>[7x]MAIAQLATEYVFSDFLLKEPTEPKFKGLRLELAVDKMVTCIAVGLPLLLISLAFAQEISIGTQISCFSPSSFSWRQAAFVDSYCWAAVQQKNSLQSESGNLPLWLHKFFPYILLLFAILLYLPPLFWRFAAAPHICSDLKFIMEELDK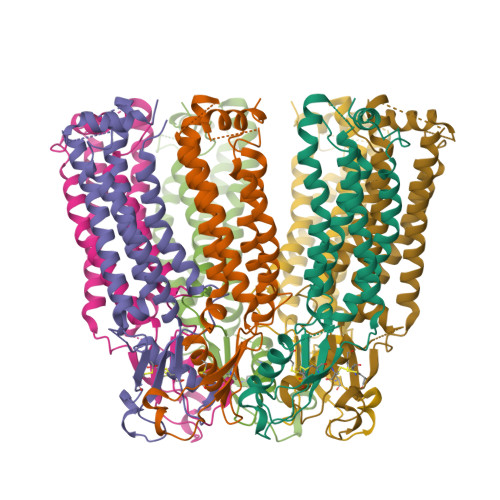VYNRAIKAAKSARDLDMRDGACSVPGVTENLGQSLWEVSESHFKYPIVEQYLKTKKNSNNLIIKYISCRLLTLIIILLACIYLGYYFSLSSLSDEFVCSIKSGILRNDSTVPDQFQCKLIAVGIFQLLSVINLVVYVLLAPVVVYTLFVPFRQKTDVLKVYEILPTFDVLHFKSEGYNDLSLYNLFLEENISEVKSYKCLKVLENIKSSGQGIDPMLLLTNLGMIKMDVVDGKTPMSAEMREEQGNQTAELQGMNIDSETKANNGEKNARQRLLDSSCSNSLEVLFQ> MNTSFGSVVPSTNFNFFKGHGNNDNTSANSTVNNSNFFLNSNETKPSKNVFMVHSTSQKKSQQPLQNLSHSPSYTENKPDKKKKYMINDAKTIQLVGPLISSPDNLGFQKRSHKARELPRFLINQEPQLEKRAFVQDPWDKANQEKMISLEESIDDLNELYETLKKMRNTERSIMEEKGLVDKADSAKDLYDAIVFQGTCLDMCPTFERSRRNVEYTVYSYEKNQPNDKKASRTKALKVFARPAAAAAPPLPSDVRPPHILVKTLDYIVDNLLTTLPESEGFLWDRMRSIRQDFTYQNYSGPEAVDCNERIVRIHLLILHIMVKSNVEFSLQQELEQLHKSLITLSEIYDDVRSSGGTCPNEAEFRAYALLSKIRDPQYDENIQRLPKHIFQDKLVQMALCFRRVISNSAYTERGFVKTENCLNFYARFFQLMQSPSLPLLMGFFLQMHLTDIRFYALRAL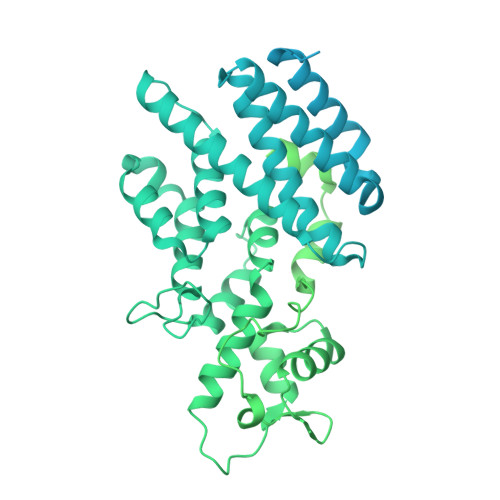SHTLNKKHKPIPFIYLENMLLFNNRQEIIEFCNYYSIEIINGDAADLKTLQHYSHKLSETQPLKKTYLTCLERRLQKTTYKGLINGGEDNLASSVYVKDPKKDRIPSIADQSFLMENFQNNYNEKLNQNSSVKPQINTSPKRVATRPNHFPFSQESKQLPQISQSHTLSTNPLLTPQVHGDLSEQKQQQIKTVTDGGSPFVFDQSAQNSTVEASKAHMISTTSNGAYDEKLSSEQEEMRKKEEQRIEEEKTQLKKKQENADKQVITEQIANDLVKEVVNSSVISIVKREFSEANYRKDFIDTMTRELYDAFLHERLYLIYMDSRAELKRNSTLKKKFFEKWQASYSQAKKNRILEEKKREEIKLVSHQLGVPGFKKSTCLFRTPYKGNVNSSFMLSSSDKNLIFSPVNDEFNKFATHLTKISKLWRPLEMQSIYYDNLTKKFPSNSLTPANLFIYAKDWTSLSNRWILSKFNLQTAQDSKKFSNNIISSRIICIDDEYEPSDFSDLQLLIFNTGVTNPDIFDLEMKLKDDGEELIKLITGISLNTNICFSLLIIYWESAENTLSESTIKHLLKLNRISKNYSSVIERIDLMNLTEESPHKCLEDKLSEISHSYVYKLTERGKYDKTLRQKRSLAGIHSRSTQLQTTKDIDQKMKKMLEKEKNKYQQQIGERNTYAHLESHIDASPRSKKRKLPILLSTSHSSQFKTPLASRLNTSGSSTSPPLPSHLAMKFRKNSRVTSLHTVLPVSTPSHSNNIPAASFSGNNTTDIQSQQLIENQKSTSVYLNNVSERILGNQEICQTPINPVTPVLDGADQGKEDIPDSILELKILIDSVKKKVNND>MASMTGGQQMGRREAGITGTWYNQLGSTFIVTAGADGALTGTYESAAGKAESRYVLTGRYDSAPATDGSGTALGWTVAWKNNYRNAHSATTWSGQYVGG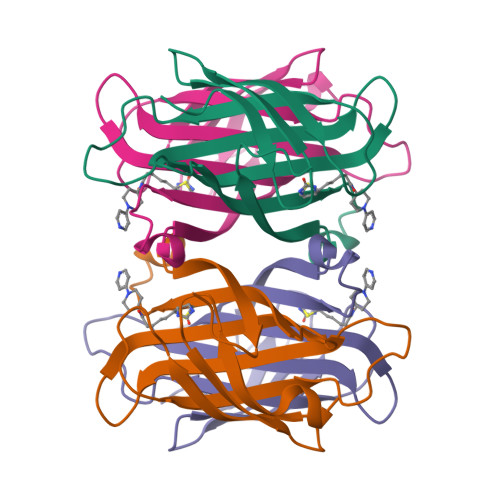AEARINTQWLLTFGATEANGWASTYVGHDTFTKVKPSAASIDAAKKAGVNNGNPLDAVQQ[2x]> GAQVSTQKTGAHETSLTASGNSTIHYTNINYYKDAASNSANRQDFTQDPSKFTEPMKDVMIKSLPALNSPTVEECGFSDRVRSITLGNSTITTQECANVVVGYGVWPSYLQDNEATAEDQPTQPDVATCRFYTLDSIQWQK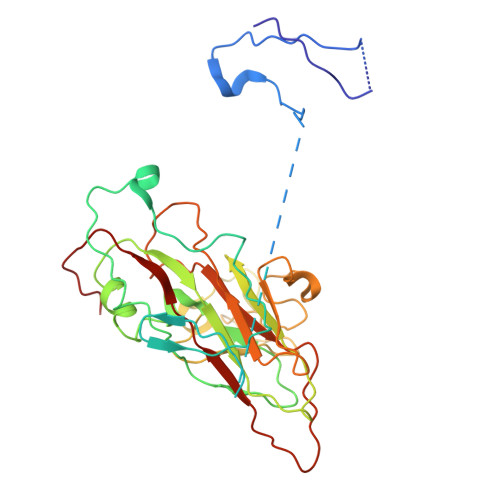ESDGWWWKFPEALKNMGLFGQNMEYHYLGRSGYTIHVQCNASKFHQGCLLVVCVPEAEMGCSDVEREVVAASLSSEDTAKSFSRTESNGQHTVQTVVYNAGMGVGVGNLTIFPHQWINLRTNNSATIVMPYINSVPMDNMFRHYNFTLMIIPFAKLEYTEQASNYVPITVTVAPMCAEYNGLRLASHQ>[4x]MYGSKTFIKYVSGIPDYFKQSFPEGFTWERTTTYEDGGFLTA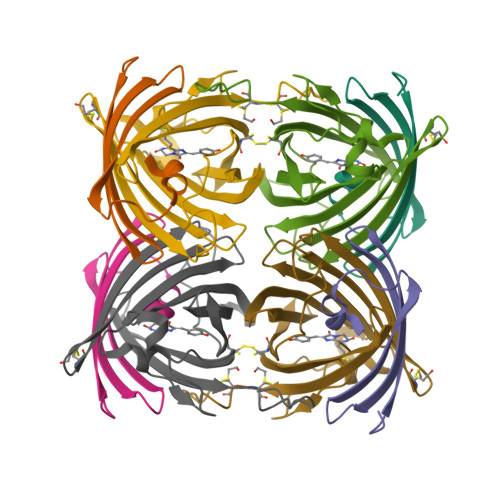HQDTSLDGDCLVYKVKILGNNFPADGPVMQNKAGGWEPGCEILYEVDGVLCGQSLMALKCPGGRHLNCRLHTTYRSKKPASALKMPEFHFEDHRIEVKEVQKGKHYEQYEAAVARYCDAAPSKLGHH;>[4x]MASLLTETMPFRMTMEGTVNGHHFKCTGKGEGNPFEGTQDMKIEVIEGGPLPFAFDILSTSC> MINRSTAFISKNLRQANLTQSSLAMKTQYNQMGFSSDNPYNKRWEYKWKHSYYTYPRDYEHTEVRKPQDSKDVPPIYFAYYKDFVDRWLPGMNMWWQRRHRIFDKFNVYFLPGMSLFFYQFADLALGFKIMAAFPLFLAYTRIRDKTLDPDFKETYLRDMIYQNPEITKYFNEETIHVLDYEFEYLPGYLCPEKFPEYQNKTWQFFNTDTAQAEGFFKFG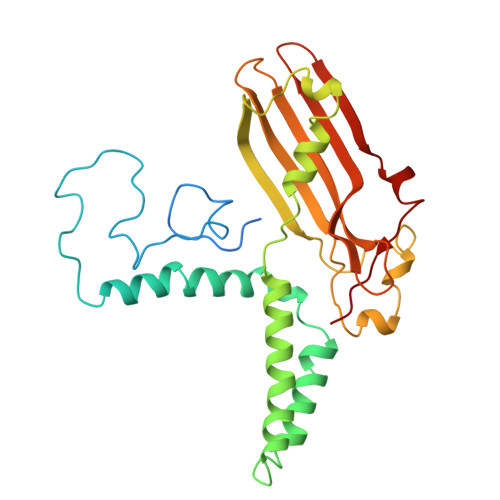DVESGATMTLKFKTMPIPGKFRYQVGEPFYFYDLRAEIKCDGVYKEVVLVDEKESLKKIRPFLFLI N-[(1S)-1-[({(1S)-3-PHENYL-1-[2-(PHENYLSULFONYL)ETHYL]PROPYL}AMINO)CARBONYL]-3-(PHENYLSULFONYL)PROPYL]MORPHOLINE-4-CARBOXAMIDE | C32 H39 N3 O7 S2 | 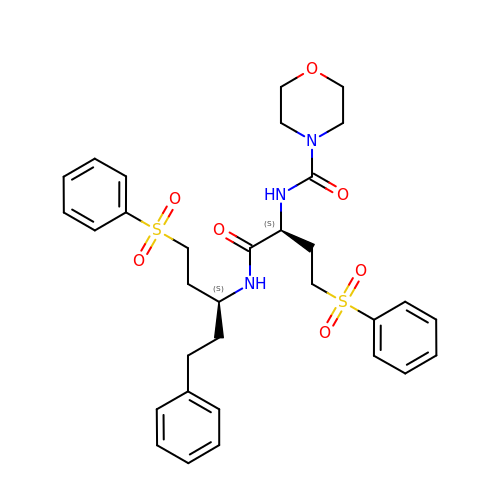UBNUVKZLXUKEGC-FIBWVYCGSA-N> STGSATTTPIDSLDDAYITPVQIGTPAQTLNLDFDTGSSDLWVFSSETTASEVDGQTIYTPSKSTTAKLLSGATWSISYGDGSSSSGDVYTDTVSVGGLTVTGQAVESAKKVSSSFTEDSTIDGLLGLAFSTLNTVSPTQQKTFFDNAKASLDSPVFTADLGYHAPGTYNFGFIDTTAYTGSITYTAV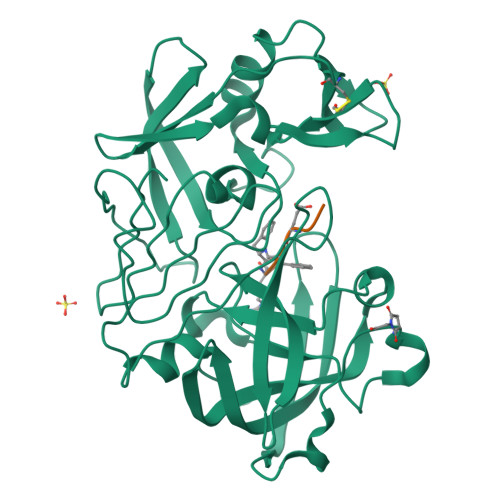STKQGFWEWTSTGYAVGSGTFKSTSIDGIADTGTTLLYLPATVVSAYWAQVSGAKSSSSVGGYVFPCSATLPSFTFGVGSARIVIPGDYIDFGPISTGSSSCFGGIQSSAGIGINIFGDVALKAAFVVFNGATTPTLGFASK;> PTEXRE> MENDMKSLSAAAQACVKKMRDAKVNEACIRTFIAQHVMVSKGETGSIPDSAIMPVDSLDALDSLTIECDNAVLQSTVVLKLNGGLGTGMGLCDAKTLLEVKDGKTFLDFTALQVQYLRQHCSEHLRFMLMDSFNTSASTKSFLKARYPWLYQVFDSEVELMQNQVPKILQDTLEPAAWAENPAYEWAPPGHGDIYTALYGSGKLQELVEQGYRYMF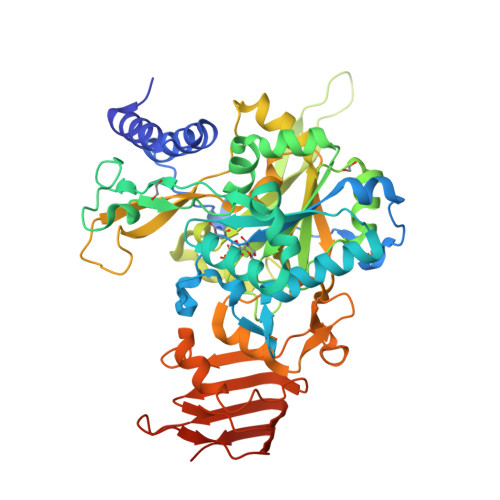VSNGDNLGATIDKRVLAYMEKEKIDFLMEVCRRTESDKKGGHLARQTVYVKGKDGQPDAEKRVLLLRESAQCPKADMESFQDINKYSFFNTNNLWIRLPVLLETMQEHGGTLPLPVIRNEKTVDSSNSASPKVYQLETAMGAAIAMFESASAIVVPRFRFAPVKTCADLLALRSDAYVVTDDFRLVLDDRCHGHPPVVDLDSAHYKMMNGFEKLVQHGVPSLVECKRVTVKGLVQFGAGNVLTGTVTIENTDSASAFVIPDGAKLNDTTASPQQSTNKMRPLEHHHHHH2-(6-hydroxy-3-oxo-3H-xanthen-9-yl)-5-[(sulfanylcarbonyl)amino]benzoic 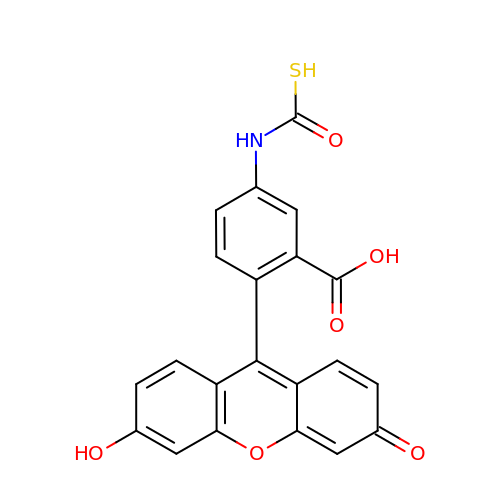acid | C21 H13 N O6 S | YMGUTVDFHHFZIJ-UHFFFAOYSA-N The hexameric low-pH stress response enzyme oxalate decarboxylase catalyzes the decarboxylation of the oxalate mono-anion in the soil bacterium Bacillus subtilis. A single protein subunit contains two Mn-binding cupin domains, and catalysis depends on Mn(III) at the N-terminal site. A π-stacked tryptophan pair (W96/W274) links two neighboring protein subunits together, thus reducing the Mn-to-Mn distance from 25.9 Å (intrasubunit) to 21.5 Å (intersubunit). The present study suggests a mechanistic function for the C-terminal Mn as an electron hole donor for the N-terminal Mn.

In order to protect the quaternary structure, we used the aromatic amino acid phenylalanine, which we hypothesized would maintain a π-stacking interaction with the neighboring indole, while disrupting the hole-hopping chain due to its higher reduction potential. However, when one of the Trp residues is replaced by Phe (W96F and W274F), the hopping time grows by a factor of 4 to 6. We also find that the vertical ionization energy (VIE) for the F96/W274 dimer is 7.19 eV (VIE for the Y96/W274 and W96/W274 dimers are 7.09 eV and 6.94 eV, respectively), thus indicating a larger energy barrier for hole transfer from the C-terminal Mn to the F96/W274 dimer. Indeed, both W→F single mutants are significantly impaired, showing only approximately 10% to 20% of the WT activity in W96F and W274F, respectively. The experimental results indicate that both W→F single mutations reduce kcat by almost two orders of magnitude. X-ray crystallography was carried out on single crystals of the W96F and W96Y forms to determine the structure of the W mutant proteins. W96F and W96Y mutants share the wildtype tertiary structure. Significantly, the π-stacking of W274 with the substituted phenylalanine (W96F) and tyrosine (W96Y) aromatic ring system was conserved. The average distance of the aromatic planes within each dimer differed only marginally by ∼ 0.1 Å or less. We therefore conclude that the loss of activity for the phenylalanine mutants is not due to a disruption of the quaternary structure.

> MKKQNDIPQPIRGDKGATVKIPRNIERDRQNPDMLVPPETDHGTVSNMKFSFSDTHNRLEKGGYAREVTVRELPISENLASVNMRLKPGAIRELHFHKEAEWAYMIYGSARVTIVDEKGRSFIDDVGEGDLWYFPSGLPHSIQALEEGAEFLLVFDDGSFSENSTFQLTDWLAHTPKEVIAANFGVTKEEISNLPGKEKYIFENQLPGSLKDDIVEGPNGEVPYPFTYRLLEQEPIESEGGKVYIADSTNFKVSKTIASALVTVEPGAMRELHWHPNTHEWQYYISGKARMTVFASDGHARTFNYQAGDVGYVPFAMGHYVENIGDEPLVFLEIFKDDHYADVSLNQWLAMLPETFVQAHLDLGKDFTDVLSKEKHPVVKKKCSK>[2x]GSDQVQKVDQYLYHMRLSDETLLEISKRFRKEMEKGLGATTHPTAAVKMLPTFVRSTPDGTEHGEFLALDLGGTNFRVLWVKVTDNGLQKVEMENQIYAIPEDIMRGSGTQLFDHIAECLANFMDKLQIKDKKLPLGFTFSFPCHQTKLDESFLVSWTKGFKSSGVEGRDVVALIRKAIQRRGDFDIDIVAVVNDTVGTMMTCGYDDHNCEIGLIVGTGSNACYMEEMRHIDMVEGDEGRMCINMEWGAFGDDGSLNDIRTEFDQEIDMGSLNPGKQLFEKMISGMYMGELVRLILVKMAKEELLFGGKLSPELLNTGRFETKDISDIEGEKDGIRKAREVLMRLGLDPTQEDCVA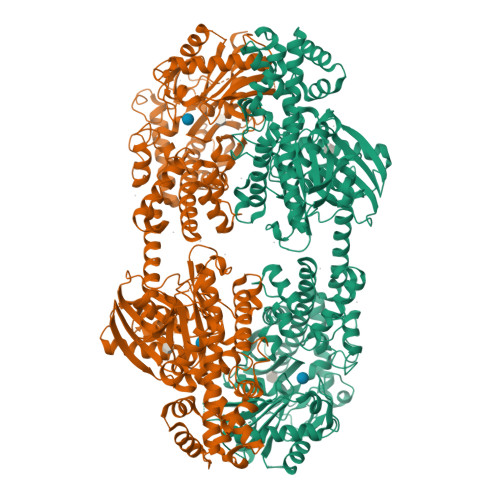THRICQIVSTRSASLCAATLAAVLQRIKENKGEERLRSTIGVDGSVYKKHPHFAKRLHKTVRRLVPGCDVRFLRSEDGSGKGAAMVTAVAYRLADQHRARQKTLEHLQLSHDQLLEVKRRMKVEMERGLSKETHASAPVKMLPTYVCATPDGTEKGDFLALDLGGTNFRVLLVRVRNGKWGGVEMHNKIYAIPQEVMHGTGDELFDHIVQCIADFLEYMGMKGVSLPLGFTFSFPCQQNSLDESILLKWTKGFKASGCEGEDVVTLLKEAIHRREEFDLDVVAVVNDTVGTMMTCGFEDPHCEVGLIVGTGSNACYMEEMRNVELVEGEEGRMCVNMEWGAFGDNGCLDDFRTEFDVAVDELSLNPGKQRFEKMISGMYLGEIVRNILIDFTKRGLLFRGRISERLKTRGIFETKFLSQIESDCLALLQVRAILQHLGLESTCDDSIIVKEVCTVVARRAAQLCGAGMAAVVDRIRENRGLDALKVTVGVDGTLYKLHPHFAKVMHETVKDLAPKCDVSFLQSEDGSGKGAALITAVACRIREAGQ>[2x]PNFSGNWKIIRSENWEELLKVLGVNVMLRKIAVAAASKPAVEIKQEGDTFYIKTSTTVRTTEINFKVGEEFEEQTVDGRPCKSLV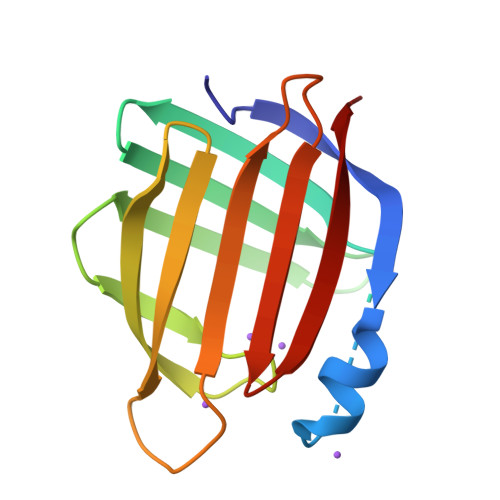KWESENKMVCEQKLLKGEGPKTSWTRELTNDGELILTMTADDVVCTRVYVRE>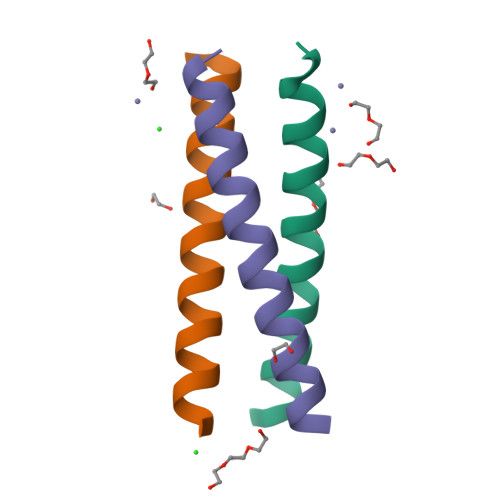XEWEALEKKLAALESKCQALEKKLEALEHGX[3x]>MREVVIVSAVRTAIGSFGGTLKDVSAVDLGAIVIKEAVKRAGIKPEQVDEVIFGNVIQAGVGQSLARQSAVYAGLPVEVPAFTVNKLCGSGLRTVSLAASLISNGDADTIVVGGSENMSASPYLIPKARFGYRMGEAKIYDAMLHDGLIDSFNNYHMGITAENIAEKWGITREDQDKFALASQQKAEAAIKAGKFKDEIVPVTVKMKKKEVVFDTDEDPRFGTTIETLAKLKPAFKRDGTGTVTAGNSSGINDSSAALILMSADKAKELGVKPMAKYVDFASAGLDPAIMGYGPYYATKKVLAKTNLTIKDFDL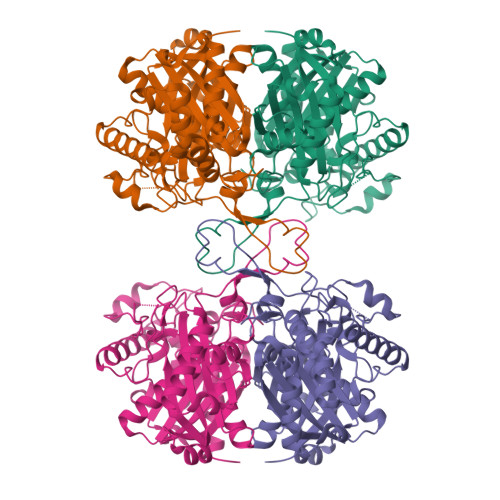IEANEAFAAQSIAVARDLEFDMSKVNVNGGAIALGHPVGCSGARILVTLLHEMQKRDAKKGLATLCIGGGQGTAVVVERLEHHHHHH[2x]>SNAMTGYLMETTLMTKHYDYLAIGGGSGGIASINRAAMYGKKCALIEAKQLGGTCVNVGCVPKKVMWHAAQIAEAIHLYGPDYGFDTTVNHFDWKKLIANRTAYIDRIHQSYERGLGNNKVDVIQGFARFVDAHTVEVNGETITADHILIATGGRPSHPDIPGAEYGIDSDGFFELDEMPKRVAVVGAGYIAVEIAGVLNGLGTETHLFVRKHAPLRTFDPLIVETLLEVMNTEGPKLHTESVPKAVIKNADGSLTLQLENGTEVTVDHLIWAIGREPATDNLNLSVTGVKTNDKGYIEVDKFQNTNVKGIYAVGDNTGVVELTPVAVAAGRRLSERLFNNKPDEHLDYSNIPTVVFSHPPIGTIGLTEPQAREKFGDDQVKVYTSSFTAMYSAVTQHRQPCRMKLVCVGAEE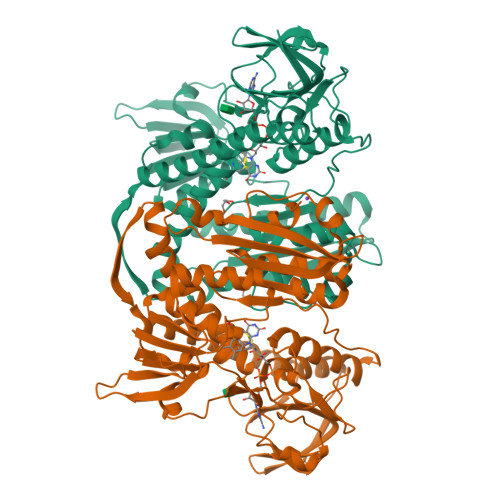KIVGIHGIGFGMDEILQGFAVAMKMGATKKDFDNTVAIHPTAAEEFVTMR[2x]2-FORMYL-6-METHOXYPHENYL DIHYDROGEN PHOSPHATE | C8 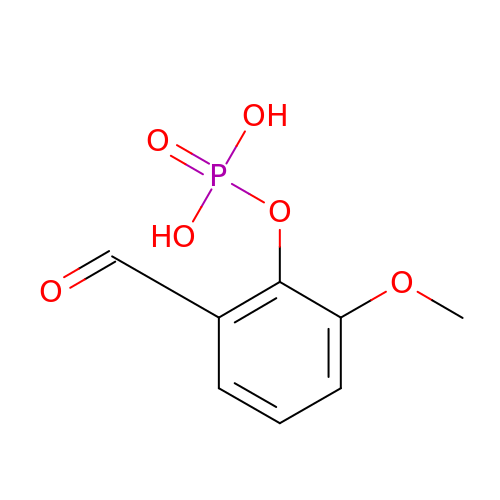H9 O6 P | CGEZBCISRKFHLZ-UHFFFAOYSA-N> PSSSMADFRKFFAKAKHIVIISGAGVSAESGVPTFRGAGGYWRKWQAQDLATPLAFAHNPSRVWEFYHYRREVMGSKEPNAGHRAIAECETRLGKQGRRVVVITQNIDELHRKAGTKNLLEIHGSLFKTRCTSCGVVAENYKSPICPALSGKGAPEPGTQDASIP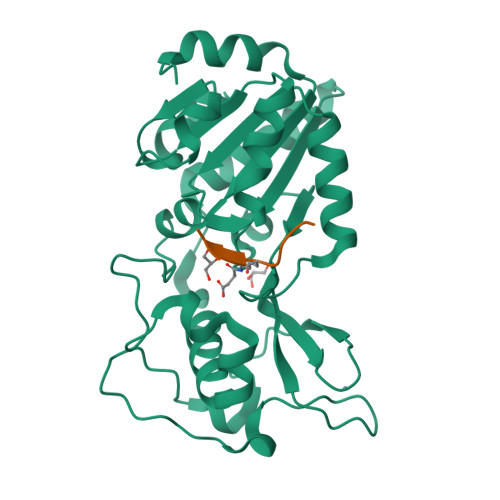VEKLPRCEEAGCGGLLRPHVVWFGENLDPAILEEVDRELAHCDLCLVVGTSSVVYPAAMFAPQVAARGVPVAEFNTETTPATNRFRFHFQGPCGTTLPEALA;> TIMPXDIQ>MLVSVYLALLVACVGQAHSQANLMRLKSDLFNRSPMYPGPTKDDPLTVTLGFFLQDIVKVDSSTNEVDLVYYERQRWKLNSLMWDPNEYGNITDFRTSAADIWTPDITAASSTRPVQVLSPQIAVVTHDGSVMFSPAQRLSFMCDPTGVDSEEGVTCAVKFESWVYSGFEIDLKTDTDQVDLSSYYASSKYEILSATQTRQVQHYSCCPEPYIDVNLVVKFRERRAGNGFFRNLFDENLYFQGHHHHHH[10x]

Protein-engineering methods have been exploited to produce a surrogate system for the extracellular neurotransmitter-binding site of a heteromeric human ligand-gated ion channel, the glycine receptor. Acetylcholine-binding protein is a highly conserved ortholog of the pLGIC extracellular ligand-binding domain (ECD) with properties similar to nAChR. Mutations affecting key residues in the orthosteric agonist site at the α1(−)/β(+) interface affect the potency of both activation by glycine and inhibition by strychnine. We therefore set out to generate a high-fidelity surrogate of this α1(−)/β(+) orthosteric binding site using the 2α1:3β stoich­iometry [Fig. 1(a)] by exploiting protein-engineering methods and the thermal stability of acetylcholine-binding protein from Aplysia californica (AcAChBP). Ultimately, the highly stable AcAChBP framework has allowed us to introduce nine amino-acid substitutions that have resulted in a stable surrogate for a heteromeric neurotransmitter site that binds glycine.

Variant II therefore reverted back to Trp164, but with the inclusion of a G162E substitution. Crystal structures of variant II with HEPES, tropisetron and strychnine revealed that the G162E substitution was accommodated with the structure essentially unperturbed compared with variant I, although now incorporating two charged residues (Arg74 and Glu162) to polarize the binding site such that the principal side is negatively charged and the complementary side is positive. The complex structure with HEPES showed this crystallization buffer component binding in two orientations in the orthosteric site in a similar fashion to that reported for LsAChBP. The variant II complex showed tropisetron [Fig. 3(a)] to be present in two of the ten orthosteric sites in the asymmetric unit, with the other sites being occupied by the cryoprotectant ethane-1,2-diol and the N-terminal histidine tails of symmetry-related molecules. The second pose is influenced by the Y110A and G162E substitutions, which allow a solvent-bridged interaction between the glutamate and tropisetron N1. van der Waals interactions between the tropane and aromatic residues are maintained in both poses with minor adjustments of side chains. The T53F substitution and the placement of the aromatic group help to place the arginine from the Q74R substitution to participate in a cation–π stacking arrangement of the guanidinyl moiety and the indole system, pushing tropisetron over towards the disulfide linkage on loop C. A solvent-mediated link between Ser135 and Arg74 may also contribute to the placement of the guanidinyl moiety. The indole N10 is directed out towards bulk solvent, whilst the carbonyl group accepts a hydrogen bond donated from the side chain of Tyr72.> MNYSLEDLPNSGKNPRVYMDIVLNNEIIGRLQIKLFRDAFPAGVENFVQLTNGKTYRVNSNGTGKYKYNRHINRTYEGCKFHNVLHNNYIVSGDIYNSNGSSAGTVYCDEPIPPVFGDYFYPHESKGLLSLVPYTDESGNRYYDSTFMITLDDIRPSNVLDELDRDQVVIGQVYGGLDVLDKINSMIKPYAGRKYPTFSIGKCGAYLDSSQAQRKRPVNVNGTKRFLNKPT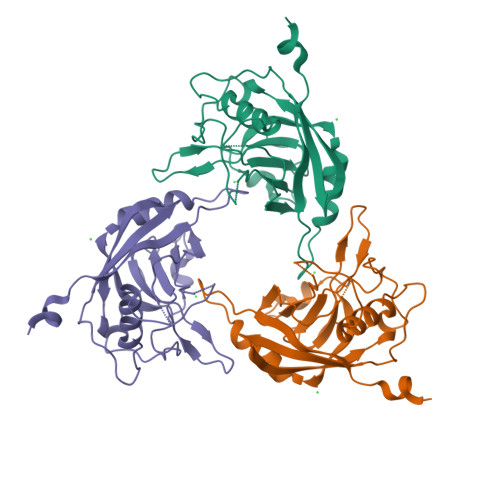RVN>[2x]MVQPSLPQDDTPDQQEQRNRAIAQQREAYQYSETAGILLIKTLPQSEMFSLKYLIERDKGLVSLIANTLASNIENIFDPFDKLEDFEEMFPLLPKPLVMNTFRNDRVFARQRIAGPNPMVIERVVDKLPDNFPVTD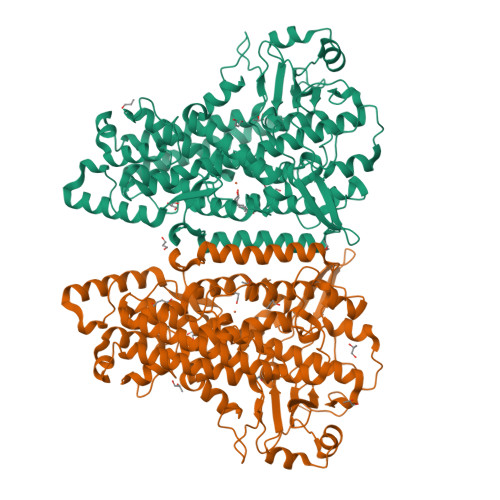AMFQKIMFTKKTLAEAIAQGKLFITNYKGLAELSPGRYEYQKNGTLVQKTKTIAAPLVLYAWKPEGFGDYRGSLAPIAIQINQQPDPITNPIYTPRDGKHWFIAKIFAQMADGNCHEAISHLARTHLILEPFVLATANELAPNHPLSVLLKPHFQFTLAINELAREQLISAGGYADDLLAGTLEASIAVIKAAIKEYMDNFTEFALPRELARRGVGIGDVDQRGENFLPDYPYRDDAMLLWNAIEVYVRDYLSLYYQSPVQIRQDTELQNWVRRLVSPEGGRVTGLVSNGELNTIEALVAIATQVIFVSGPQHAAVNYPQYDYMAFIPNMPLATYATPPNKESNISEATILNILPPQKLAARQLELMRTLCVFYPNRLGYPDTEFVDVRAQQVLHQFQERLQEIEQRIVLCNEKRLEPYTYLLPSNVPNSTSI>[2x]MTKWVLHVDLDQFYASVELRRRPDLRGQPVIVGGSGDPSEPRKVVTCASYEAREFGVHAGMPLRAAARRCPDATFLPSDPAAYDEASEQVMGLLRDLGHPLEVWGWDEAYLGADLPDESDPVEVAERIRTVVAAETGLSCSVGISDNKQRAKVATGFAKPAGIYVLTEANWMTVMGDRPPDALWGVGPKTTKKLAAMGITTVADLAVTDPSVLTT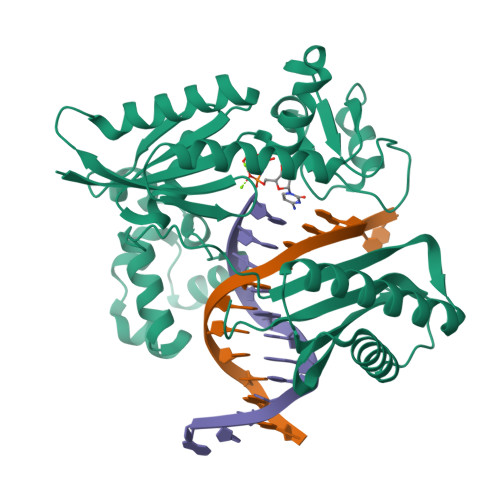AFGPSTGLWLLLLAKGGGDTEVSSEPWVPRSRSHVVTFPQDLTERREMDSAVRDLALQTLAEIVEQGRIVTRVAVTVRTSTFYTRTKIRKLPAPSTDAGQIVDTALAVLDQFELDRPVRLLGVRLELAMDDVPRPAVTAGT>AAUUGAAAAAUCAAUAGAUUUAAACCUAGUGAAGAGCAUUUGAACAAUGUGCUAGGGUAGUAUGGGAUAAGUCGAUAACUAAAAUGAAUUGGGAUACUGAUUGAUUUUAGUGGUGGAUUUUACAGCAAUGUAAAAAGGACUAAUAGUAAAAGCUAUUAAUCGCAAAGUACUACGUGGAAUUUGUGCAGGUGUAAGGUACGAAACUUUCGAGUGUGACAAUAGACGCUCCAGUGGAGAAUAAUCUAAGUUAGGUGGAAGUGUGAGAAGCUUGGCAGACCUUAGAAAACUCAAACCAAGCGCUUUGCAGAGAAACUGAGAAAUCAGUGUUUAACGAAAGAAGUCGGUACGAGUAGCUUAAUGCAGCAAUUUAUUUACAGAUGACAAAUAAUAAAAAUGGGACUCUUAUGUAAAUGCUGAAUGUUCAAGUGAAAGUUAUUAGCCAGUAGAGCUAGAUCAUACAGAAAAAGCAAAGAGAAGCUAUUGGGUAGCGCCCGAUAGUUCAGCCUCUUUGGGUAUGUGACUGAAUAACACUGUAAACAAAGGAAGCAGGAAGAAA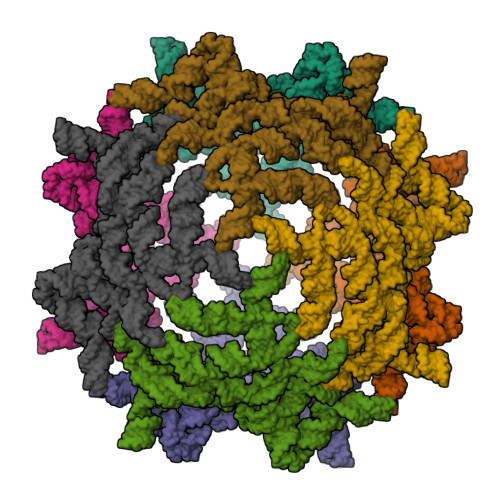AGCCUAAAUCUGUUGAUUUUUGAG[8x]>CGAAXUCG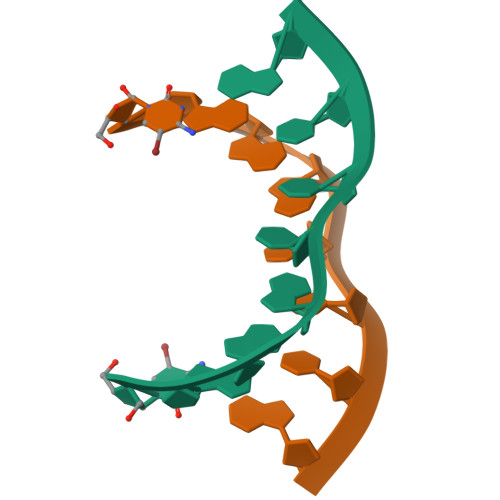[8x]>SHPALTQLRALRYCKEIPALDPQLLDWLLLEDSMTKRFEQQGKTVSVTMIREGFVEQNEIPEELPLLPKESRYWLREILLCADGEPWLAGRTVVPVSTLSGPELALQKLGKTPLGRYLFTSSTLTRDFIEIGRDAGLWGRRSR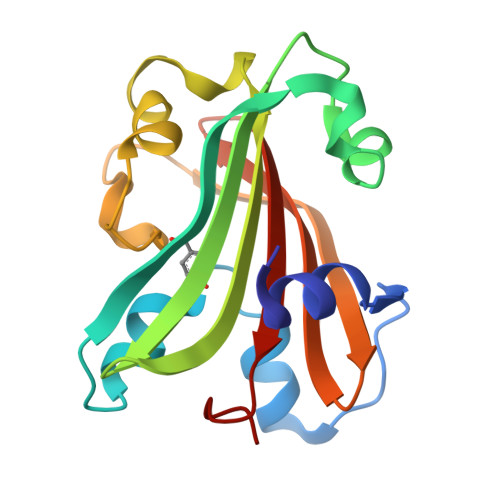LRLSGKPLLLTELFLPASPLY[2x]2-[3-[(1~{R})-1-[(2~{S})-1-[(2~{S})-2-cyclohexyl-2-(3,4,5-trimethoxyphenyl)ethanoyl]piperidin-2-yl]carbonyloxy-3-(3,4-dimethoxyphenyl)propyl]phenoxy]ethanoic acid | C42 H53 N O11 | 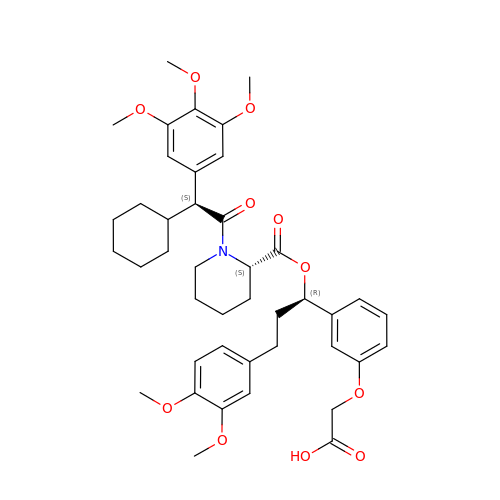OEQZPFWOEOOISR-AKTKKGGCSA-N>MGSDKIHHHHHHENLYF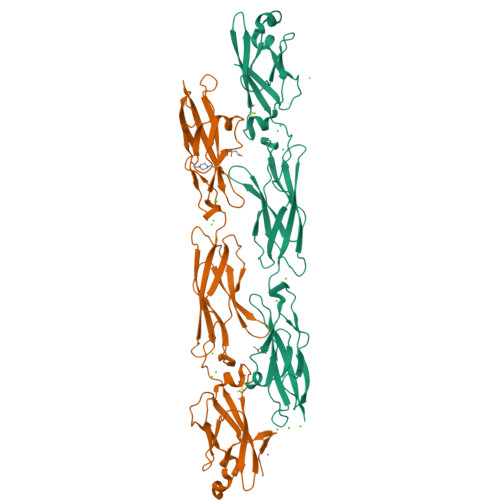QGSTIIHYEILEERERGFPVGNVVTDLGLDLGSLSARRLRVVSGASRRFFEVNWETGEMFVNDRLDREELCGTLPSCTVTLELVVENPLELFSAEVVVQDINDNNPSFPTGEMKLEISEALAPGTRFPLESAHDPDVGSNSLQTYELSHNEYFALRVQTREDGTKYAELVLERALDWEREPSVQLVLTALDGGTPARSATLPIRITVLDANDNAPAFNQSLYRARVREDAPPGTRVAQVLATDLDEGLNGEIVYSFGSHNRAGVRELFALDLVTGVLTIKGRLDFEDTKLHEIYIQAKDKGANPEGAHCKVLVEVVD[2x]> WTPFSWVEKYAYAFSGPYNKAEVALTFDDGPDLEFTPKILDKLKQHNVKATFFLLGENAEK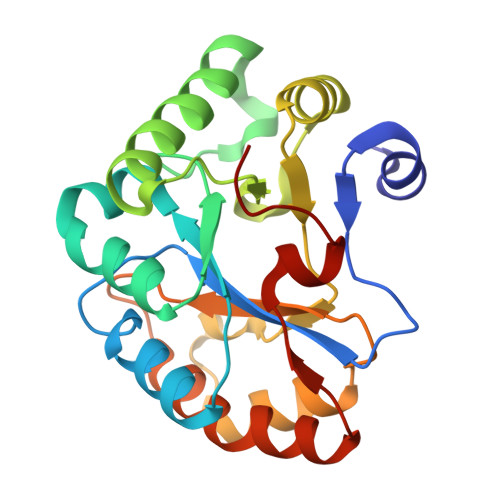FPNIVKRIANEGHVIGNHTYSHPNLAKVNEDEYRNQIIKTEEILNRLAGYAPKFIRPPYGEILENQLKWATEQNFMIVQWSVDTVDWKGVSADTITNNVLGNSFPGSVILQHSTPGGHLQGSVDALDKIIPQLKTKGARFVTLPSMFQTSKER> HHHHHHGGCRPSAQSLEIKHGDLSINSANNHYAAQTLSVSCDVPANIRFMLLRNTTPTYSHGKKFSVGLGHG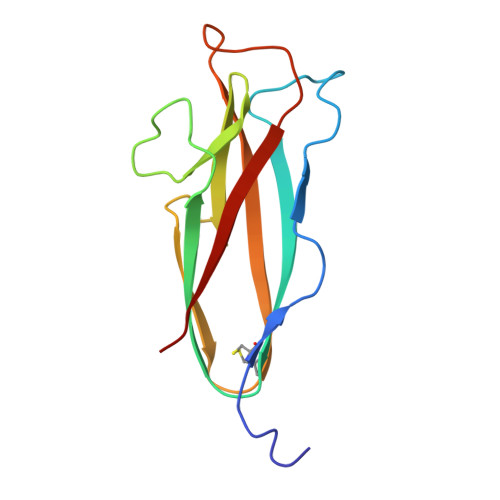WDSIVSVNGVDTGETTMRWYKAGTQNLTIGSRLYGESSKIQPGVLSGSATLLMILP> ARRAVAVLRGDAGVSGIIYFQQGSGGSITTISGSVSGLTPGLH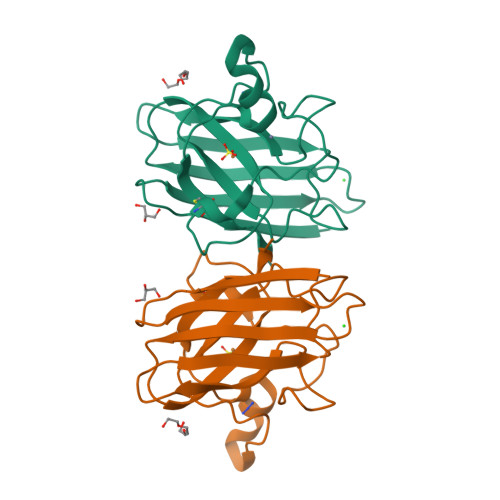GFHVHQYGDQTNGCTSAGDHYNPFGKTHGGPNDRIKHIGDLGNIVAGANGVAEVYINSYDIKLRGPLSVIGHSLVVHANTDDLGQGTGNMREESLKTGNAGSRLACGVIGIAAVS1,3-BIS-([3-[3-[3-(4-{3-[3-NITRO-5-(GALACTOPYRANOSYLOXY)-BENZOYLAMINO]-PROPYL}-PIPERAZIN-1-YL)-PROPYLAMINO-3,4-DIOXO-CYCLOBUTENYL]-AMINO-PROPOXY-ETHOXY-ETHOXY]-PROPYL-]AMINO-CARBONYLOXY)-2-AMINO-PROPANE 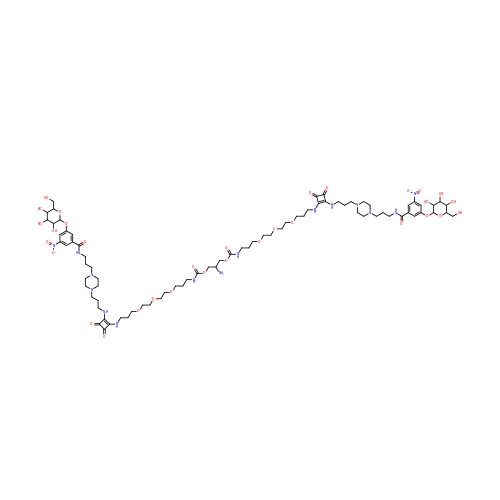| C79 H123 N15 O32 | BPHYTQORKHDHAH-OHNHNXIVSA-N>GSAMARKRIITPEKKELIRNLISEYNITSAKDLQEALKDLLGDTIQNMLEAELDEHLGYEKYESTEEAKSNYRNGYTSKTLKSSVGQVEIDIPRDRNAEFEPKIVPRYKRDISEIENKIIAMYARGMSTREINEQIQEIYGFEVSAEMVSKITDKILPEIEEWQKRPLGEVYPIVFIDAIHFSVKNDGIVGKKAVYIVLAIDIEGQKDVIGIYVGENESSKFWLSVLNDLKNRGVKDILILCADALSGIKDAINAAFPNTEYQRCIVHQIRNTLKYVSDKDRKEFARDLKRIYTAPNEKAGYDQMLEVSEKWEKKYPAAMKSWKSNWDVICPFFKYSEELRKIMYTTNTIESLNSSYRRINKSRTVFPGDQSLLKSIYLATVKITSKWTMRYKNWGLILGQLQIMFEGRI[2x]

Copy‐out/paste‐in transposition is a major bacterial DNA mobility pathway. The pre‐reaction complex (PRC) is a complex of TnpA with DNA representing the first 26 bp of the R‐TIR with six flanking bp (fR‐TIR26); the pre‐cleaved complex (PCC) is a complex with the first 26 bp of the R‐TIR (R‐TIR26); and strand transfer complex 1 (STC1) is a complex with oligonucleotide R26(j6)L15‐5′rec in which a 6‐bp bridging spacer links two TIRs and is an approximation of the Figure‐eight intermediate. In all three complexes, a single DNA molecule is bound by a dimer of TnpA and they are all remarkably asymmetric. In each structure, the R‐TIR is recognized through an extensive protein–DNA interface in which almost all of the interactions are contributed by one protomer (“A”) with the exception of the transposon tip which is directed toward the catalytic domain (“CD”; residues 165–261 + 325–407) of the second protomer (“B”), suggesting that catalysis occurs in trans.

The PRC structure captures the binding state before the initial nicking step on the donor TIR, where we observed TnpA interacting with both the donor TIR and flanking DNA. In the PRC, representing the state in which the flanking sequence is still present and before any chemical step has occurred, the transposon tip is away from the active site of CDB as helix α9 of the ID is inserted in the major groove at the flanking region (1–5 base pairs from the TIR end), where it interacts with the DNA through K280, R284, K287, and R288. The scissile phosphate in fR‐TIR26 is displaced ~ 8 Å from the position of the R‐TIR26 3′‐OH in the PCC structure and ~ 16 Å from the equivalent position of the scissile phosphate in Hermes when bound to DNA (Hickman et al, 2018). Although the resolution of the structures is limited and none of them contains metal ions in the active sites, in the PCC and PRC, the side chains of D175 and D241 are in the appropriate conformation for metal binding and catalysis whereas the side chain of E348 is pointing away from the presumed metal‐binding site. When we superimposed the A protomers of the PCC and PRC structures (which can be done with an overall r.m.s.d. of ~ 1.1 Å over 400 Cα positions), the clear difference is a ~ 6 Å change in the position of IDB as it closes down on the transposon end in the absence of the flanking sequence. The inherent mobility of the ID is supported by a normal mode analysis using iMODS (López‐Blanco et al, 2014) in the absence of DNA which indicated that the ID can move relative to the CD. Furthermore, the primary mode of ID motion is consistent with the motion seen in the comparison of the two complex structures. The structures and the iMODS analysis suggest that the relative flexibility of the ID and CD domains may be key to a conformation change that transiently places the transposon end in the trans‐active site of CDB.> MLHRTRLAQLINGRILQYFVPYERDEVNPVVFMDVTVEGDALGRVSVELFHDIVPKTTENFRSLCTGERGYSQCPLFYKGIPFHRVIPGFIVQGGDILLKDGRGNVSVFGFPFPDESFEGKAGKHLRGTVAMAHSAPNQNGSQFFFNLARNDHLDGKFVVCGQVIDGWEVVDRVAVLSGSSCGTPVSRAWITECGQSSGD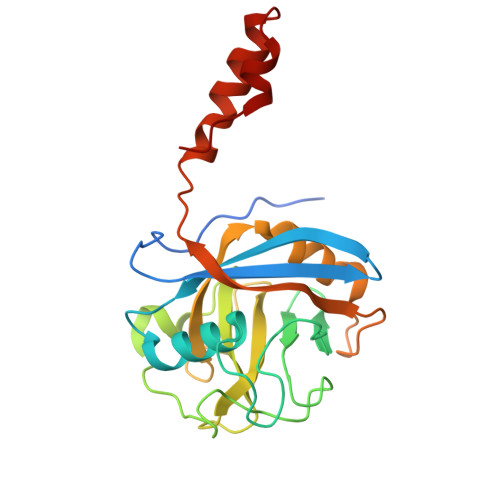KLEDTERALSGERALHTMPGKEVLDILSPRY>[6x]MSSAIKEVQGAPVKWVTNWTPEAIRGLVDQEKGLLDPRIYADQSLYELELERVFGRSWLLLGHESHVPETGDFLATYMGEDPVVMVRQKDKSIKVFLNQCRHRGMRICRSDAGNAKAFTCSYHGWAYDIAGKLVNVPFEKEAFCDKKEGDCGFDKAEWGPLQARVATYKGLVFANWDVQAPDLETYLGDARPYMDVMLDRTPAGTVAIGGMQKWVIPCNWKFAAEQFCSDMYHAGTTTHLSGILAGIPPEMDLSQAQIPTKGNQFRAAWGGHGSGWYVDEPGSLLAVMGPKVTQYWTEGPAAELAEQRLGHTGMPVRRMVGQHMTIFPTCSFLPAMNQIRVWHPRG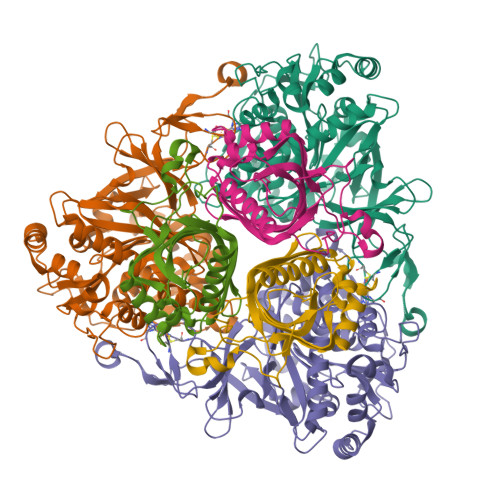PNEIEVWAFTLVDADAPAEIKEEYRRHNIRNFSAGGVFEQDDGENWVEIQKGLRGYKAKSQPFNAQMGLGRSQTGHPDFPGNVGYVYAEEAARGMYHHWMRMMSEPSWATLKP;>[6x]MTNPSPHFFKTFEWPSKAAGLELQNEIEQFYYREAQLLDHRAYEAWFALLDKDIHYFMPLRTNRMIREGELEYSGDQDLAHFDETHETMYGRIRKVTSDVGWAENPPSRTRHLVSNVIVKETATPDTFEVNSAFILYRNRLERQVDIFAGERRDVLRRADNNLGFSIAKRTILLDASTLLSNNLSMFF> MAFYSCCWVLLALTWHTSAYGPDQRAQKKGDIILGGLFPIHFGVAAKDQDLKSRPESVECIRYNFRGFRWLQAMIFAIEEINSSPALLPNLTLGYRIFDTCNTVSKALEATLSFVAQNKIDSLNLDEFCNCSEHIPSTIAVVGATGSGVSTAVANLLGLFYIPQVSYASSSRLLSNKNQFKSFLRTIPNDEHQATAMADIIEYFRWNWVGTIAADDDYGRPGIEKFREEAEERDICIDFSELISQYSDEEEIQHVVEVIQNSTAKVIVVFSSGPDLEPLIKEIVRRNITGKIWLASEAWASSSLIAMPQYFHVVGGTIGFALKAGQIPGFREFLKKVHPRKSVHNGFAKEFWEETFNCHLQEGAKGPLPVDTFLRGHEESGDRFSQSSTAFRPLCTGDENINSVETPYIDYTHLRISYNVYLAVYSIAHALQDIYTCLPGRGLFTNGSCADIKKVEAWQVLKHLRHLNFTNNMGEQVTFDECGDLVGNYSIINWHLSPEDGSIVFKEVGYYNVYAKKGERLFINEEKILWSGFSREVPFSNCSRDCLAGTRKGIIEGEPTCCFECVECPDGEYSDETDASACNKCPDDFWSNENHTSCIAKEIEFLSDYKDDDDK

The extracellular calcium-sensing receptor (CaSR) is responsible for the maintenance of a stable blood Ca2+ level. CaSR is a class C G-protein-coupled receptor (GPCR). Ligand binding to CaSR takes place within a large extracellular Venus Flytrap (VFT) module that consists of two domains (LB1 and LB2). In addition, CaSR contains a cysteine-rich (CR) domain that connects the VFT module to the transmembrane region.

Form I crystal structure of CaSR ECD represents the inactive configuration since the VFT modules of both protomers are in the open conformation associated with the resting state (open-open), and the interdomain cleft is empty. In addition, each protomer structure contains one Ca2+ ion and three SO42- ions. The inactive structure of CaSR ECD shows that subunit association in the resting state is primarily mediated by the LB1 domains. In the inactive homodimer, only minimal contacts occur between the LB2 domains. The inactive structure revealed electron density at site 2 that is consistent with a bound Ca2+ ion. The inactive and active structures share a common Ca2+-binding mode at site 2, suggesting that the bound Ca2+ is an integral part of the CaSR structure. In the inactive structure, electron densities revealed that anions were bound at sites 1–3. The anion at site 1 is coordinated by the guanidine group of R62 and backbone nitrogen of Y63. Second, the anions at sites 1 and 3 appear to stabilize the inactive conformation. Binding of anions at these sites prevent favorable interactions across the interdomain cleft that promote VFT closure.>AEAGITGTWYNQLGSTFIVTAGADGALTGTYESAVGNAESRYVLTGRYDS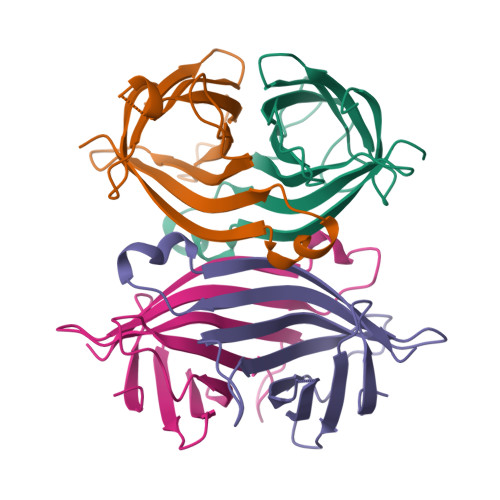APATDGSGTALGWTVAWKNNYRNAHSATTWSGQYVGGAEARINTQFLLTSGTTEANAWKSTLVGHDTFTKVKPSAAS[4x]> ADTIVAVELDTYPN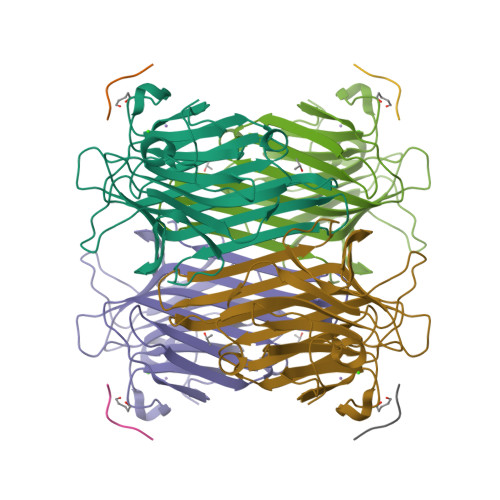TDIGDPSYPHIGIDIKSVRSKKTAKWNMQNGKVGTAHIIYNSVDKRLSAVVSYPNADSATVSYDVDLDNVLPEWVRVGLSASTGLYKETNTILSWSFTSKLKSNSTHETNALHFMFNQFSKDQKDLILQGDATTGTDGNLELTRVSSNGSPQGSSVGRALFYAPVHIWESSAVVASFEATFTFLIKSPDSHPADGIAFFISNIDSSIPSGSTGRLLGLFPDAN;> MYWYPY>MKKLQIAVGIIRNENNEIFITRRAADAHMANKLEFPGGKIEMGETPEQAVVRELQEEVGITPQHFSLFEKLEYEFPDRHITLWFWLVERWEGEPWGKEGQPGEWMSLVGLNADDFPPANEPV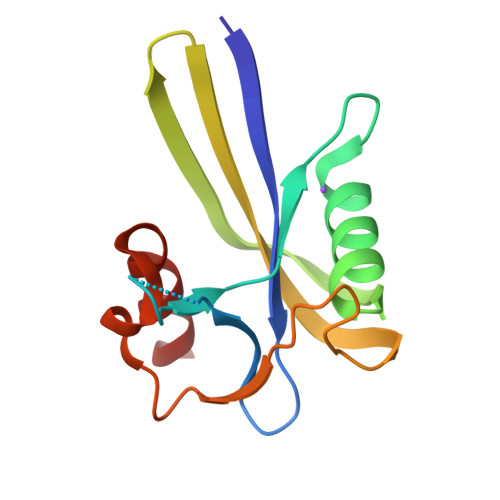IAKLKRL[2x]>[2x]AGHMTSILSRNHVKVKGSGKASIMFAPGFGCDQSVWNAVAPAFEEDHRVILFDYVGSGHSDLRAYDLNRYQTLDGYAQDVLDVCEALDLKETVFVGHSVGALIGMLASIRRPELFSHLVMVGPS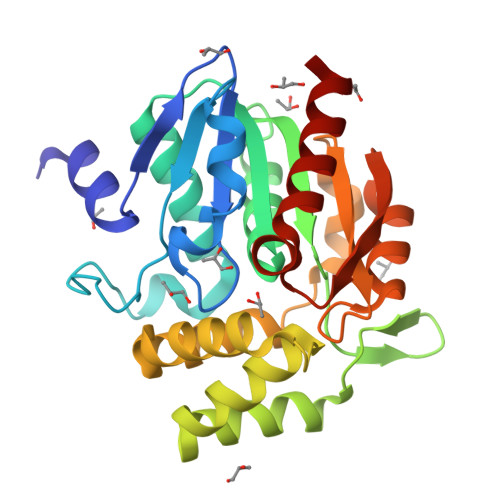PCYLNDPPEYYGGFEEEQLLGLLEMMEKNYIGWATVFAATVLNQPDRPEIKEELESRFCSTDPVIARQFAKAAFFSDHREDLSKVTVPSLILQCADDIIAPATVGKYMHQHLPYSSLKQMEARGHCPHMSHPDETIQLIGDYLKAHV>MHHHHHHGSTSLYKKAGSETLYIQGDHLPMPKFGPLAGLRVVFSGIEIAGPFAGQMFAEWGAEVIWIENVAWADTIRVQPNYPQLSRRNLHALSLNIFKDEGREAFLKLMETTDIFIEASKGPAFARRGITDEVLWQHNPKLVIAHLSGFGQYGTEEYTNLPAYNTIAQAFSGYLIQNGDVDQPMPAFPYTADYFSGLTATTAALAALHKVRETGKGESIDIAMYEVMLRMGQYFMMDYFNGGEMCPR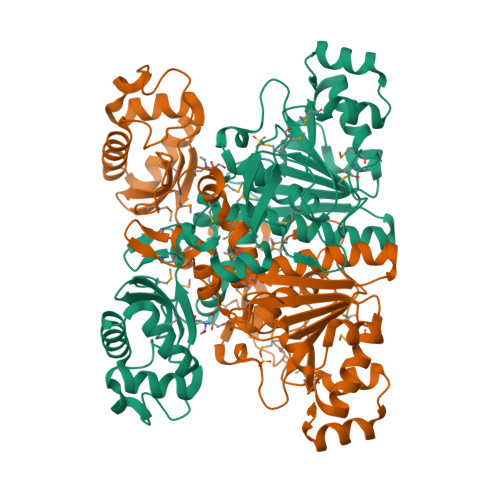MSKGKDPYYAGCGLYKCADGYIVMELVGITQIEECFKDIGLAHLLGTPEIPEGTQLIHRIECPYGPLVEEKLDAWLATHTIAEVKERFAELNIACAKVLTVPELESNPQYVARESITQWQTMDGRTCKGPNIMPKFKNNPGQIWRGMPSHGMDTAAILKNIGYSENDIQELVSKGLAKVEDSTHHHHHH[2x]>[3x]MNPFHELEPGPEVPEVVYALIEIPKGSRNKYELDKKTGLLKLDRVLYSPFFYPVDYGIIPQTWYDDGDPFDIMVIMREPVYPLTIIEARPIGIMKMEDSGDKDWKVLAVPVEDPYFNDWK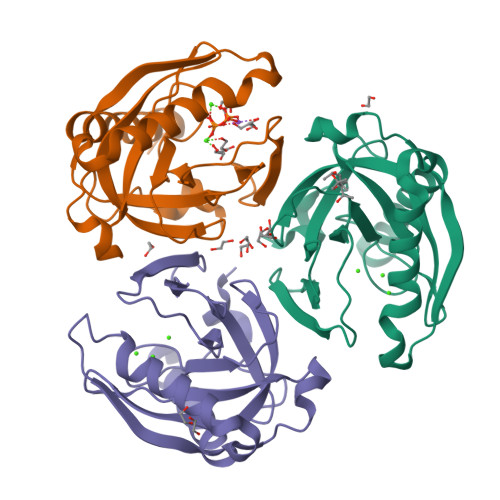DISDVPKAFLDEIAHFFQRYKELQGKTTKIEGWGNAEEAKREILRAIEMYKEKFGKEE> EFRHDSRKIPKVGHTFFQKPESCPPVPGGSMKLDIGIINENQRVSMSRNIESRSTSPWNYTVTWDPNRYPSEVVQAQCRNLGCINAQGKEDISMNSVPIQQETLVVRR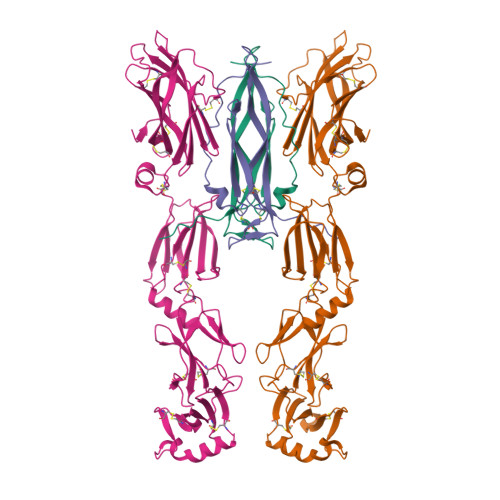KHQGCSVSFQLEKVLVTVGCTCVTPVIHHVQ;> LERLVGPQDATHCSPGLSCRLWDSDILCLPGDIVPAPGPVLAPTHLQTELVLRCQKETDCDLCLRVAVHLAVHGHWEEPEDEEKFGGAADSGVEEPRQASLQAQVVLSFQAYPTARCVLLEVQVPAALVQFGQSVGSVVYDCFEAALGSEVRIWSYTQPRYEKELQHTQQLPDCRGLEVWNSIPSCWALPWLQVSADGDNVHLVLQVSEEQHFGLSLYWNQVQGPPKPRWHKNLTGPQIITLQHTDLVPCLCIQVWPLEPDSVRTNICPFREDPRAHQNLWQAARLRLLTLQSWLLDAPCSLPAEAALCWRAPGGDPCQPLVPPLSWEQVTVDKVLEFPLLKGHPNLCVQVQSSEKLQLQECLWADSLGPLKDDVLLLETRGPQDQRSLCALEPSGCTSLPSKASTRAARLGEYLLQDLQSGQCLQLWDDDLGALWACPMDKYIHKREFRH> HGTTANTHCGADFCTWWHDSGEINTQTPVQPGNVRQSHKYSVQVSLAGTNNFHDSFVYESIPRNGNGRIYAPTDPPNSNTLDSSVDDGISIEPSIGLNMAWSQFEYSHDVDVKILATDGSSLGSPSDVVIRPVSISYAISQSDDGGIVIRVPADANGRKFSVEFKTDLYTFLSDGNEYVTSGGSVVGVEPTNALVIFASPFLPSGMIPHMTPDNTQTMTPGPINNGDWGAKSILYFPPGVYWMNQDQSGNSGKLGS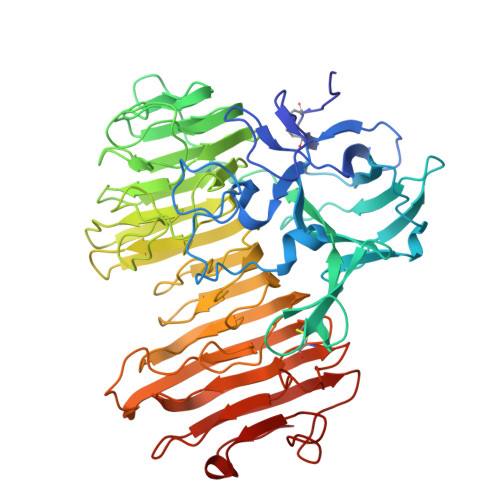NHIRLNSNTYWVYLAPGAYVKGAIEYFTKQNFYATGHGILSGENYVYQANAGDNYIAVKSDSTSLRMWWHNNLGGGQTWYCVGPTINAPPFNTMDFNGNSGISSQISDYKQVGAFFFQTDGPEIYPNSVVHDVFWHVNDDAIKIYYSGASVSRATIWKCHNDPIIQMGWTSRDISGVTIDTLNVIHTRYIKSETVVPSAIIGASPFYASGMSPDSRKSISMTVSNVVCEGLCPSLFRITPLQNYKNFVVKNVAFPDGLQTNSIGTGESIIPAASGLTMGLAISAWTIGGQKVTMENFQANSLGQFNIDGSYWGEWQIS> RTSTIMTDYNPNYSFAGKTSSISDLKEVPRKNITLIRGLGHGAFGEVYEGQVSGMPNDPSPLQVAVKTLPEVCSEQDELDFLMEALIISKLNHQNIVRCIGVSLQSLPRFILLELMAGGDLKSFLRETRPRPSQPSSLAMLDLLHVARDIACGCQYLEENHFIHRDIAARNCLLTCPGPGRVAKIGDFGMARDIYR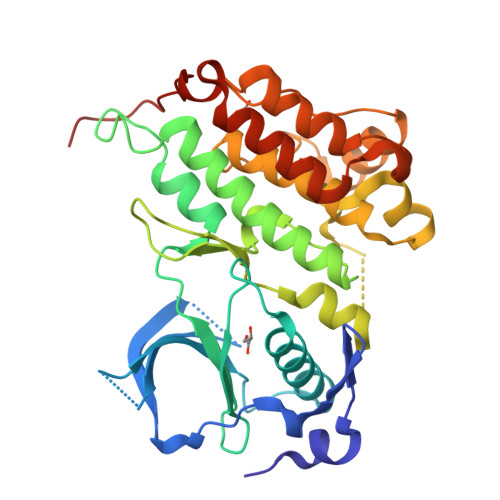ASYYRKGGCAMLPVKWMPPEAFMEGIFTSKTDTWSFGVLLWEIFSLGYMPYPSKSNQEVLEFVTSGGRMDPPKNCPGPVYRIMTQCWQHQPEDRPNFAIILERIEYCTQDPDVINTALPIEYGPLVEEEEK>MKEFYLTVEQIGDSIFERYIDSNGRERTREVEYKPSLFAHCPESQATKYFDIYGKPCTRKLFANMRDASQWIKRMEDIGLEALGMDDFKLAYLSDTYNYEIKYDHTKIRVANFDIEVTSPDGFPEPSQAKHPIDAITHYDSIDDRFYVFDLLNSPYGNVEEWSIEIAAKLQEQGGDEVPSEIIDKIIYMPFDNEKELLMEYLNFWQQKTPVILTGWNVESFAIPYVYNRIKNIFGESTAKRLSPHRKTRVKVIENMYGSREIITLFGISVLDYIDLYKKFSFTNQPSYSLDYISEFELNVGKLKYDGPISKLRESNHQRYISYNIIAVYRVLQIDAKRQFINLSLDMGYYAKIQIQSVFSPIKTWDAIIFNSLKEQNKVIPQGRSHPVQPYPGAFVKEPIPNRYKYVMSFDLTSLYPSIIRQVNISPETIAGTFKVAPLHDYINAVAERPSDVYSCSPNGMMYYKDRDGVVPTEITKVFNQRKEHKGYMLAAQRNGEIIKEALHNPNLSVDEPLDVDYRFDFSDEIKEKIKKLSAKSLNEMLFRAQRTEVAGMTAQINRKLLINSLYGALGNVWFRYYDLRNATAITTFGQMALQWIERKVNEYLNEVCGTEGEAFVLYGDTDSIYVSADKIIDKVGESKFRDTNHWVDFLDKFARERMEPAIDRGFREMCEYMNNKQHLMFMDREAIAGPPLGSKGIGGFWTGKKRYALNVWDMEGTRYAEPKLKIMGLETQKSSTPKAVQKALKECIRRMLQEGEESLQEYFKEFEKEFRQLNYISIASVSSANNIAKYDVGGFPGPKCPFHIRGILTYNRAIKGNIDAPQVVEGEKVYVLPLREGNPFGDKCIAWPSGTEITDLIKDDVLHWMDYTVLL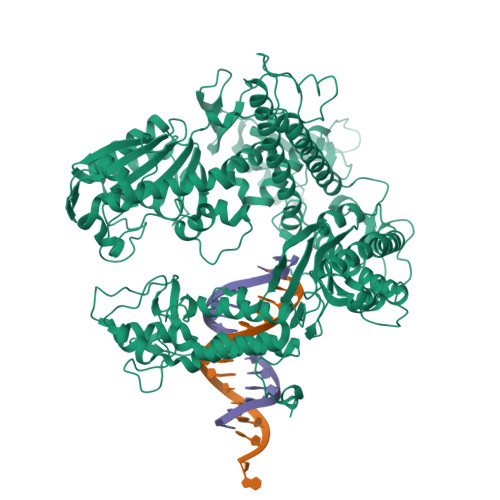EKTFIKPLEGFTSAAKLDYEKKASLFDMFDFHHH[4x]5-{2-[2-(2-oxo-4-sulfanylidene-3,4-dihydropyrimidin-1(2H)-yl)ethoxy]phenoxy}naphthalene-2-carbonitrile | C23 H17 N3 O3 S | 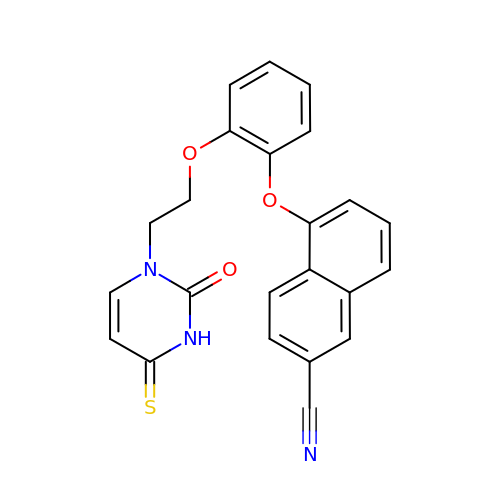MADLNJACUUKLRV-UHFFFAOYSA-N1-[3-(7,8-dihydro-5~{H}-[1,3]dioxolo[4,5-g]isoquinolin-6-ylmethyl)phenyl]-3,3-diethyl-azetidine-2,4-dione 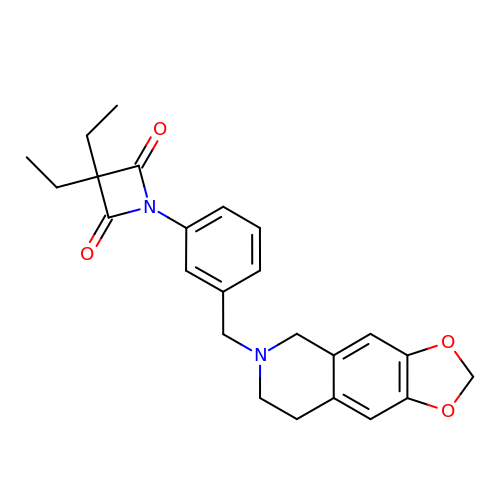| C24 H26 N2 O4 | MFVPPSBYBIAVQH-UHFFFAOYSA-N> GLIVDTRDVEERVHVARKTKLAPTVAHGVFNPEFGPAALSNKDPRLNEGVVLDEVIFSKHKGDTKMSAEDKALFRRCAADYASRLHSVLGTANAPLSIYEAIKGVDGLDA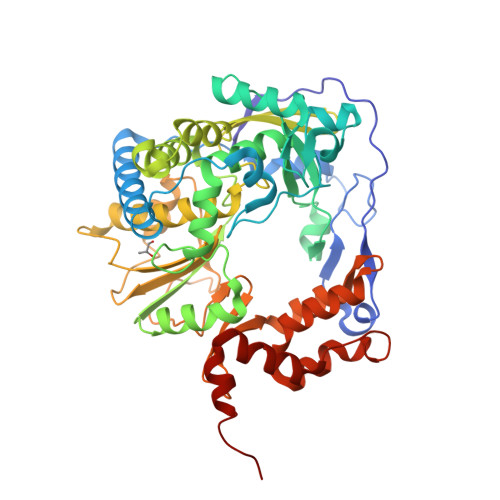MEPDTAPGLPWALQGKRRGALIDFENGTVGPEVEAALKLMEKREYKFACQTFLKDEIRPMEKVRAGKTRIVDVLPVEHILYTRMMIGRFCAQMHSNNGPQIGSAVGCNPDVDWQRFGTHFAQYRNVWDVDYSAFDANHCSDAMNIMFEEVFRTEFGFHPNAEWILKTLVNTEHAYENKRITVEGGMPSGCSATSIINTILNNIYVLYALRRHYEGVELDTYTMISYGDDIVVASDYDLDFEALKPHFKSLGQTITPADKSDKGFVLGHSITDVTFLKRHFHMDYGTGFYKPVMASKTLEAILSFARRGTIQEKLISVAGLAVHSGPDEYRRLFEPFQGLFEIPSYRSLYLRWVNAVCGDAAAALEHHHHHH>[6x]MKLPTNLAYERSIDPSDVCFFVVWPDDRKTPLTYNSRTLLGQMEAASLAYDVSGQPIKSATAEALAQGNPHQVDFCHVPYGASHIECSFSVSFSSELRQPYKCNSSKVKQTLVQLVELYETKIGWTELATRYLMNICNGKWLWKNTRKAYCWNIVLTPWPWNGEKVGFEDIRTNYTSRQDFKNNKNWSAIVEMIKTAFSSTDGLAIFEVRATLHLPTNAMVRPSQVFTEKESGSKSKSKTQNSRVFQSTTIDGERSPILGAFKTGAAIATIDDWYPEATEPLRVGRFGVHREDVTCYRHPSTGKDFFSILQQAEHYIEVLSANKTPAQETINDMHFLMANLIKGGMFQHKGD;> MQTLKELIASNPDDLTTELKRAFRPLTPHIAIDGNELDALTILVNLTDKTDDQKDLLDRAKCKQKLRDEKWWASCINCVNYRQSHNPKFPDIRSEGVIRTQALGELPSFLLSSSKIPPYHWSYSHDSKYVNKSAFLTNEFCWDGEISCLGELLKDADHPLWNTLKKLGCSQKTCKAMAKQLADITLTTINVTLAPNYLTQISLPDSDTSYISLSPVASLSMQSHFHQRLQDENRHSAITRFSRTTNMGVTAMTCGGAFRMLKSGAKFSSPPHHRLNSKRSWLTSEHVQSLKQYQRLNKSLIPENSRIALRRKYKIELQNMVRSWFAMQDHTLDSNILIQHLNHDLSYLGATKR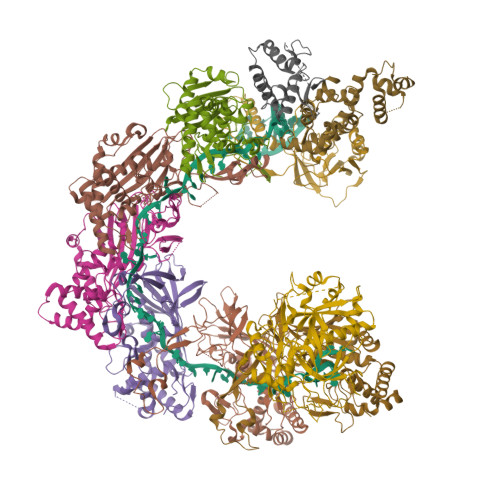FAYDPAMTKLFTELLKRELSNSINNGEQHTNGSFLVLPNIRVCGATALSSPVTVGIPSLTAFFGFVHAFERNINRTTSSFRVESFAICVHQLHVEKRGLTAEFVEKGDGTISAPATRDDWQCDVVFSLILNTNFAQHIDQDTLVTSLPKRLARGSAKIAIDDFKHINSFSTLETAIESLPIEAGRWLSLYAQSNNNLSDLLAAMTEDHQLMASCVGYHLLEEPKDKPNSLRGYKHAIAECIIGLINSITFSSETDPNTIFWSLKNYQNYLVVQPRSINDETTDKSSL;> MKWYYKTITFLPELCNNESLAAKCLRVLHGFNYQYETRNIGVSFPLWCDATVGKKISFVSKNKIELDLLLKQHYFVQMEQLQYFHISNTVLVPEDCTYVSFRRCQSIDKLTAAGLARKIRRLEKRALSRGEQFDPSSFAQKEHTAIAHYHSLGESSKQTNRNFRLNIRMLSEQPREGNSIFSSYGLSNSENSFQPVPLI;>MFLQRPKPYSDESLESFFIRVANKNGYGDVHRFLEATKRFLQDIDHNGYQTFPTDITRINPYSAKNSSSARTASFLKLAQLTFNEPPELLGLAINRTNMKYSPSTSAVVRGAEVFPRSLLRTHSIPCCPLCLRENGYASYLWHFQGYEYCHSHNVPLITTCSCGKEFDYRVSGLKGICCKCKEPITLTSRENGHEAACTVSNWLAGHESKPLPNLPKSYRWGLVHWWMGIKDSEFDHFSFVQFFSNWPRSFHSIIEDEVEFNLEHAVVSTSELRLKDLLGRLFFGSIRLPERNLQHNIILGELLCYLENRLWQDKGLIANLKMNALEATVMLNCSLDQIASMVEQRILKPNRKSKPNSPLDVTDYLFHFGDIFCLWLAEFQSDEFNRSFYVSRW[2x]>[12x]MGESERSEAFGIPRDSPLSSGDAAELEQLRREAAVLREQLENAVGSHAPTRSARDIHQLEARIDSLAARNSKLMETLKEARQQLLALREEVDRLGQPPSGYGVLLATHDDDTVDVFTSGRKMRLTCSPNIDAASLKKGQTVRLNEALTVVEAGTFEAVGEISTLREILADGHRALVVGHADEERVVWLADPLIAEDLPDGLPEALNDDTRPRKLRPGD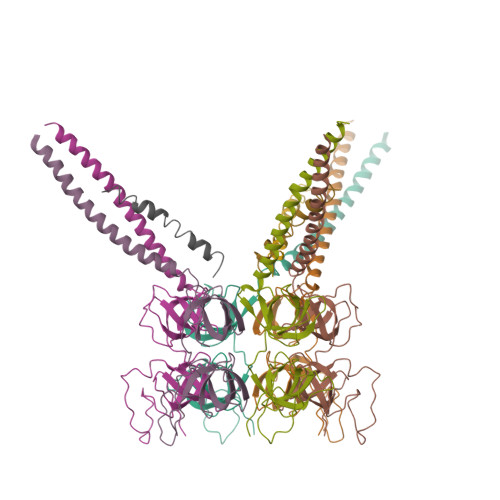SLLVDTKAGYAFERIPLVPRGSAAALEHHHHHH;>GSHMMAQEQTKRGGGGGDDDDIAGSTAAGQERREKLTEETDDLLDEIDDVLEENAEDFVRAYVQKGGE[6x]>MVDQATLDKLEAGFKKLQEASDCKSLLKKHLTKDVFDSIKNKKTGMGATLLDVIQSGVENLDSGVGIYAPDAESYRTFGPLFDPIIDDYHGGFKLTDKHPPKQWGDINTLVGLDPAGQFIISTRVRCGRSLQGYPFNPCLTAEQYKEMEEKVSSTLSSMEDELKGTYYPLTGMSKATQQQLIDDHFLFKEGDRFLQTANACRYWPTGRGIFHNDAKTFLVWVNEEDHLRIISMQKGGDLKTVYKRLVTAVDNIES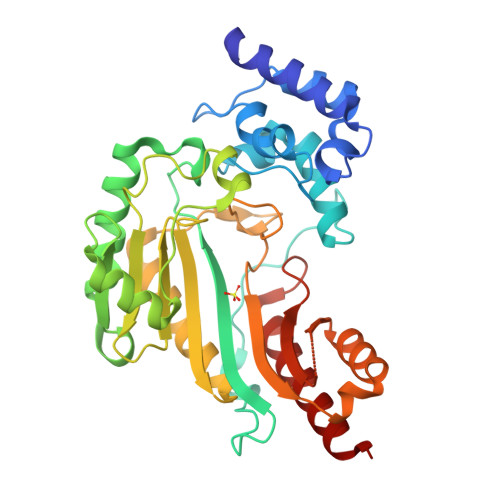KLPFSHDDRFGFLTFCPTNLGTTMRASVHIQLPKLAKDRKVLEDIASKFNLQVRGTRGEHTESEGGVYDISNKRRLGLTEYQAVREMQDGILEMIKMEKAAA[2x]>GAMGSMWKRSEQMKIKSGKCNMAAAMETEQLGVEIFETADCEENIESQDRPKLEPFYVERYSWSQLKKLLADTRKYHGYMMAKAPHDFMFVKRNDPDGPHSDRIYYLAMSGENRENTLFYSEIPKTINRAAVLMLSWKPLLDLFQATLDYGMYSREEELLRERKRIGTVGIASYDYHQGSGTFLFQAGSGIYHVKDGGPQGFTQQPLRPNLVETSCPNIRMDPKLCPADPDWIAFIHSNDIWISNIVTREERRLTYVHNELANMEEDARSAGVATFVLQEEFDRYSGYWWCPKAETTPSGGKILRILYEENDESEVEIIHVTSPMLETRRADSFRYPKTGTANPKVTFKMSEIMIDAEGRIIDVIDKELIQPFEILFEGVEYIARAGWTPEGKYAWSILLDRSQTRLQIVLISPELFIPVEDDVMERQRLIESVPDSVTPLIIYEETTDIWINIHDIFHVFPQSHEEEIEFIFASECKTGFRHLYKITSILKESKYKRSSGGLPAPSDFKCPIKEEIAITSGEWEVLGRHGSNIQVDEVRRLVYFEGTKDSPLEHHLYVVSYVNPGEVTRLTDRGYSHSCCISQHCDFFISKYSNQKNPHCVSLYKLSSPEDDPTCKTKEFWATILDSAGPLPDYTPPEIFSFESTTGFTLYGMLYKPHDLQPGKKYPTVLFIYGGPQVQLVNNRFKGVKYFRLNTLASLGYVVVVIDNRGSCHRGLKFEGAFKYKMGQIEIDDQVEGLQYLASRYDFIDLDRVGIH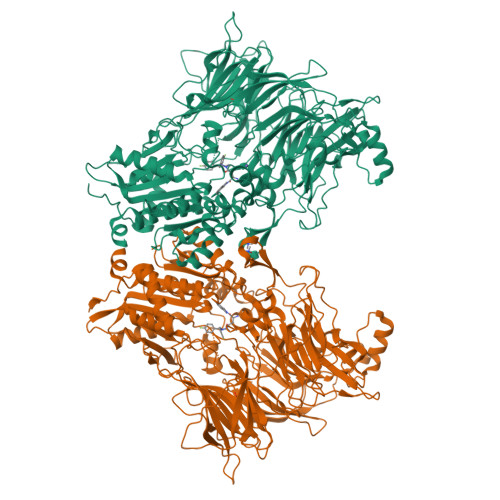GWSYGGYLSLMALMQRSDIFRVAIAGAPVTLWIFYDTGYTERYMGHPDQNEQGYYLGSVAMQAEKFPSEPNRLLLLHGFLDENVHFAHTSILLSFLVRAGKPYDLQIYPQERHSIRVPESGEHYELHLLHYLQENLGSRIAALKVI[3x]> MSEAADVERVYAAMEEAAGLLGVACARDKIYPLLSTFQDTLVEGGSVVVFSMASGRHSTELDFSISVPTSHGDPYATVVEKGLFPATGHPVDDLLADTQKHLPVSMFAIDGEVTGGFKKTYAFFPTDNMPGVAELSAIPSMPPAVAENAELFARYGLDKVQMTSMDYKKRQVNLYFSELSAQTLEAESVLALVRELGLHVPNELGLKFCKRSFSVYPTLNWETGKIDRLCFAVISNDPTLVPSS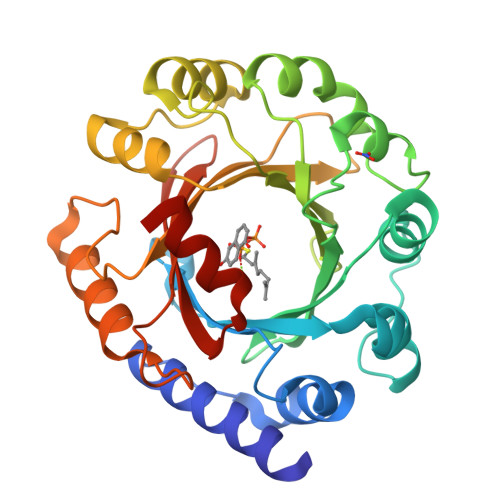DEGDIEKFHNYATKAPYAYVGEKRTLVYGLTLSPKEEYYKLGAYYHITDVQRGLLKAFDSLED>[8x]MRDPFMEALGLKVLHLAPGEAVVAGEVRADHLNLHGTAHGGFLYALADSAFALASNTRGPAVALSCRMDYFRPLGAGARVEARAVEVN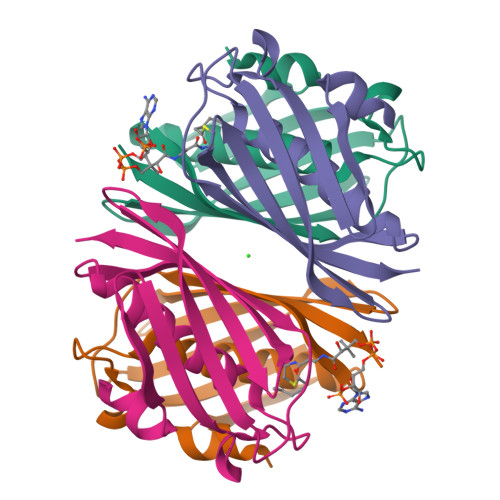LSRRTATYRVEVVSEGKLVALFTGTVFRLGGDGDDVPAGTGNLAPREA> MTDVDKRKIKIILNGEMEEAELHMITSPNRHCCLKIFHNNNQLAESNDTDYFSCFADLRNQLKNIIFLCKGAKINVYPSAMSRDMSDGIVAYETTLGQPGLPENQVHIFDFEDKYVDITPEEQRKFHSQWFESLVDHHHHHH;> MAGGIGNKGDYIITYRGDTRSFTEIFDKGFETLGPSKDLYKHALDNRAPPSDFVSTTIDPTKTISFATKYGQKSGYMYTMKTNHGIDVNKALGARSPFAAEAEIAMPGGVRAEDILGARAVNADGEMWDYTILNPKRYGK;> GASSDKIIHLTDDSFDTDVLKADGAILVDFWAEWCGPCKMIAPILDEIADEYQGKLTVAKLNIDQNPGTAPKYGIRGIPTLLLFKNGEV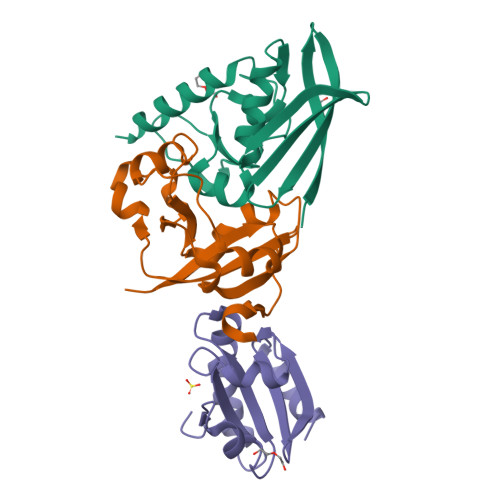AATKVGALSKGQLKEFLDANLA>GMSLANQIDQFLGTIMQFAENKHEILLGKAESDVKLTSTQEAILMLLAEQISTNAKIAEKLKISPAAVTKALKKLQEQELIKS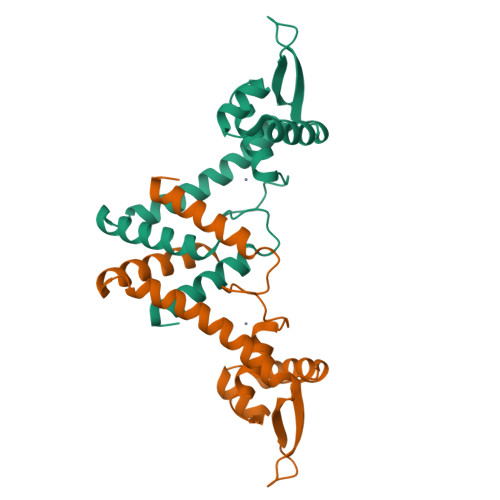SRATNDERVVLWSLTEKAVPVAKEHATHHEKTLSTYQELGNKFTDEEQEVISKFLSALTEEFQ[4x]> YFQGMLKNIDPALNADVLHALRAMGHGDTLVISDTNFPSDSVARQTTVGKVLHIDNVSAARAMKAILSVLPLDTPLQPSVGRMEVMGAPDQLEPVQVEVQQEIDAAEGKSAPMYGIERFA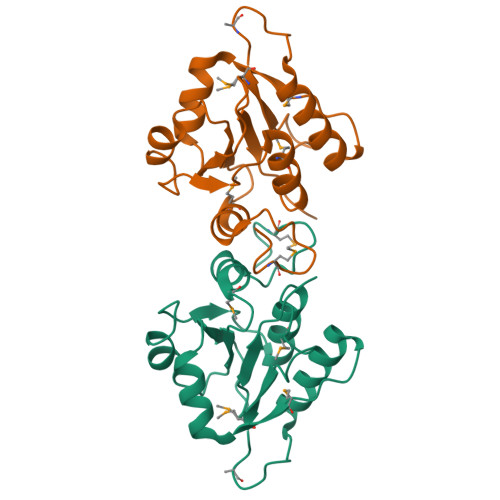FYEKAKQAYCVITTGETRFYGCFLLTKGVIPPK> SASSSDSDLSDFASSVLAEHNKKRALHKDTPALSWSDTLASYAQDYADNYDCSGTLTHSGGP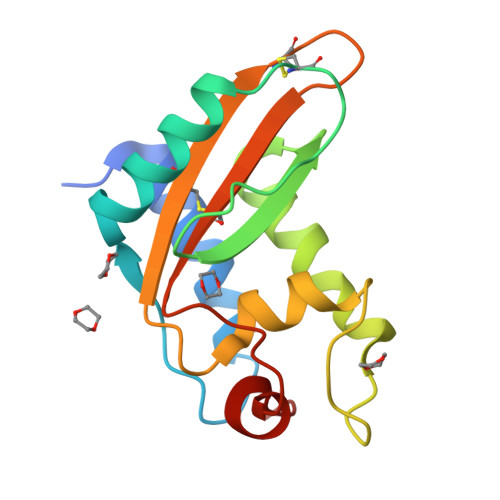YGENLALGYDGPAAVDAWYNEISNYDFSNPGFSSNTGHFTQVVWKSTTQVGCGIKTCGGAWGDYVICSYDPAGNYEGEYADNVEPLA> MMNPLIIKLGGVLLDSEEALERLFSALVNYRESHQRPLVIVHGGGCVVDELMKGLNLPVKKK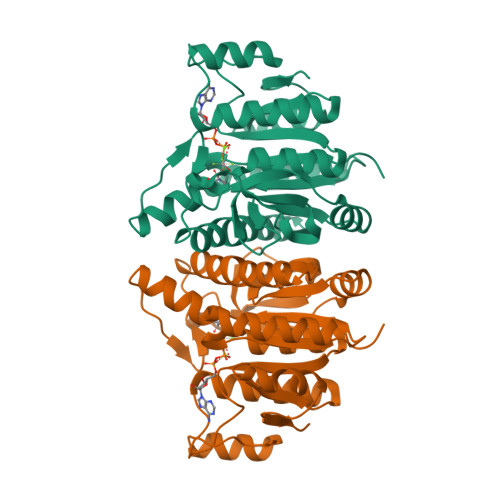NGLRVTPADQIDIITGALAGTANKTLLAWAKKHQIAAVGLFLGDGDSVKVTQLDEELGHVGLAQPGSPKLINSLLENGYLPVVSSIGVTDEGQLMNVNADQAATALAATLGADLILLSDVSGILDGKGQRIAEMTAAKAEQLIEQGIITDGMIVKVNAALDAARTLGRPVDIASWRHAEQLPALFNGMPMGTRILA>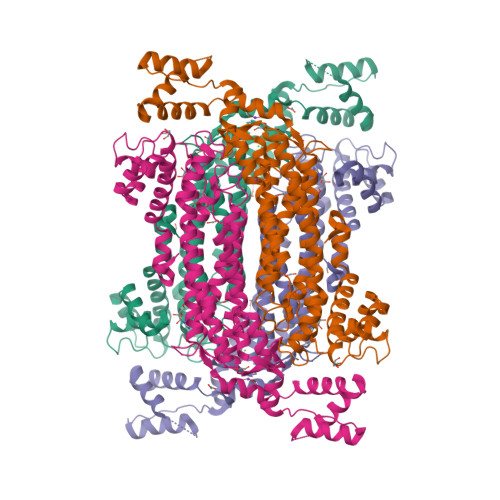[2x]MIKRYDVAEISKIWADENKYAKMLEVELAILEALEDRMVPKGTAAEIRARAQIRPERVDEIEKVTKHDIIAFCTSIAEQFTAETGKFFHFGVTSSDIIDSALSLQIRDSMSYVIKDLEALCDSLLTKAEETKEIITMGRSHGMFAEPMSFGQKFLGAYVEFKRRLKDLKDFQKDGLTVQFSGAVGNYCILTTEDEKKAADILGLPVEEVSTQVIPRDRIAKLISIHGLIASAIERLAVEIRHLHRSDVFEVYEGFSKGQKGSSTMPHKKNPISTENLTGMARMLRSHVSIALENCVLWHERDISHSSAERFYLPDNFGIMVYALRRMKNTIDNLVVQRDIIEDRVRSTSAYLSSFYLHFLVANTPFMREDCYKIVQQVAFDLKQGESFSKKLQKVMHDEHNIILDIPEMDFEGIKKTYLKEIDHVFDRSVKARGENLY> MSEYLKALFELKELRQKFIFTLLMFVIYRLGSHIPIPGINPEALRDFLKAFEGSVFALYDIFSGGNLGRLTVFALGVMPYISASIMMQLLTVAIPSLQRLAKEEGDYGRYKINEYTKYLTLFVATVQSLGIAFWIRGQVSPKGIPVVENPGISFILITVLTLVAGTMFLVWIADRITEKGIGNGASLIIFAGIVANFPNAVIQFYEKVKTGDIGPLTLLLIIALIIAIIVGIVYVQEAERRIPIQYPGRQVGRQLYAGRKTYLPIKINPAGVIPIIFAQALLLIPSTLLNFVQNPFIKVIADMFQPGAIFYNFLYVTFIVFFTYFYTAVLINPVELAENLHKAGAFIPGVRPGQDTVKYLERIINR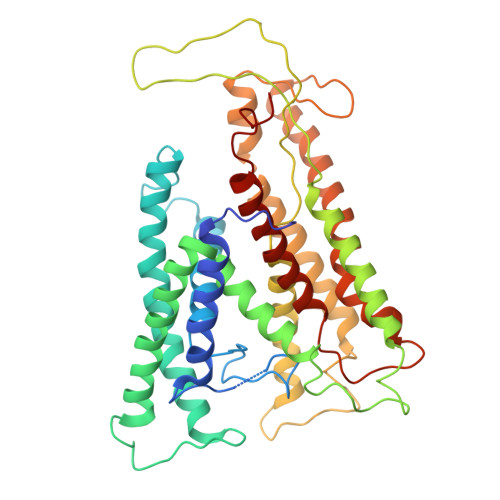LIFFGALFLSVIALIPILISVWFNIPFYFGGTTALIVVGVALDTFRQIETYLIQKKYKSYVRR>GSMSSASTFGQNAWLVDEMFQQFQKDPKSVDKEWRELFEAQGGPNTTPATTEAQPSAPKESAKPAPKAAPAAKAAPRVETKPADKTAPKAKESSVPQQPKLPEPGQTPIRGIFKSIAKNMDISLEIPTATSVRDMPARLMFENRAMVNDQLKRTRGGKISFTHIIGYAMVKAVMAHPDMNNSYDVIDGKPTLIVPEHINLGLAIDLPQKDGSRALVVAAIKETEKMNFSEFLAAYEDIVARSRKGKLTMDDYQGVTVSLTNPGGIGTRHSVPRLTKGQGTIIGVGSMDYPAEFQGASEDRLAELGVGKLVTITSTYDHRVIQGAVSGEFLRTMSRLLTDDSFWDEIFDAMNVPYTPMRWAQDVPNTGVDKNTRVMQLIEAYRSRGHLIADTNPLSWVQPGMPVPDHRDLDIETHNLTIWDLDRTFNVGGFGGKETMTLREVLSRLRAAYTLKVGSEYTHILDRDERTWLQDRLEAGMPKPTQAEQKYILQKLNAAEAFENFLQTKYVGQKRFSLEGAEALIPLMDSAIDTAAGQGLDEVVIGMPHRGRLNVLFNIVGKPLASIFNEFEGQMEQGQIGGSGDVKYHLGSEGQHLQMFGDGEIKVSLTANPSHLEAVNPVMEGIVRAKQDYLDKGVDGKTVVPLLLHGDAAFAGLGIVPETINLAKLRGYDVGGTIHIVVNNQIGFTTTPDSSRSMHYATDYAKAFGCPVFHVNGDDPEAVVWVGQLATEYRRRFGKDVFIDLVCYRLRGHNEADDPSMTQPKMYELITGRETVRAQYTEDLLGRGDLSNEDAEAVVRDFHDQMESVFNEVKEGGKKQAEAQTGITGSQKLPHGLETNISREELLELGQAFANTPEGFNYHPRVAPVAKKRVSSVTEGGIDWAWGELLAFGSLANSGRLVRLAGEDSRRGTFTQRHAVAIDPATAEEFNPLHELAQSKGNNGKFLVYNSALTEYAGMGFEYGYSVGNEDSIVAWEAQFGDFANGAQTIIDEYVSSGEAKWGQTSKLILLLPHGYEGQGPDHSSARIERFLQLCAEGSMTVAQPSTPANHFHLLRRHALSDLKRPLVIFTPKSMLRNKAAASAPEDFTEVTKFQSVINDPNVADAAKVKKVMLVSGKLYYELAKRKEKDGRDDIAIVRIEMLHPIPFNRISEALAGYPNAEEVLFVQDEPANQGPWPFYQEHLPELIPNMPKMRRVSRRAQSSTATGVAKVHQLEEKQLIDEAFEA[6x]

Contrary to most organisms in which three enzymes compose the 2-oxoglutarate dehydrogenase complex (ODH), actinobacteria rely on a two-in-one protein (OdhA) in which both the oxidative decarboxylation and succinyl transferase steps are carried out by the same polypeptide. Here we describe high-resolution cryo-EM and crystallographic snapshots of representative enzymes from Mycobacterium smegmatis and Corynebacterium glutamicum, showing that OdhA is an 800-kDa homohexamer that assembles into a three-blade propeller shape. The obligate trimeric and dimeric states of the acyltransferase and dehydrogenase domains, respectively, are critical for maintaining the overall assembly, where both domains interact via subtle readjustments of their interfaces. Schematic illustration of the reaction steps involved in the oxidative decarboxylation of 2-oxoglutarate with generation of succinyl-CoA and NADH/H+ (ODH reaction), with emphasis on the catalytic steps catalyzed by OdhA. These include the ThDP-dependent decarboxylation of the 2-oxoglutarate substrate followed the reductive acylation of the lipoyl group provided by E2p (both catalyzed by the OdhA E1o domain), and the transfer of the succinyl moiety to the CoASH acceptor (catalyzed by the OdhA E2o domain).

The same grid preparation strategy was then applied to other full-length OdhA samples, i.e. enzyme without added ligands, or preincubated with either CoASH or succinyl-CoA, leading to maps at comparable resolutions of 2.1-2.2 Å. In all cases, the maps, which showed well-defined density for most side chains, allowed to trace the OdhA polypeptide chain unambiguously starting from residue Pro102, corresponding to the N-terminal boundary of the E2o domain, with excellent stereochemical parameters. In contrast, the full N-terminal OdhA segment, corresponding to the first hundred residues that include a predicted helical hairpin analogous to the one observed in the crystal structure of MsKGD, could not be traced due to the lack of supporting density, confirming its high mobility in solution. The E1o active site at the dimer interface showed a clear density for ThDP-Mg2+ in all cases. In contrast to the crystallographic structure of OdhAΔ97 which fits the resting state, all our models refined on single particle EM maps adopt an activated conformational state of the E1o domain, even in the absence of added ligands. The state is indeed revealed by the shifts in the loops 566-579 as well as 809-836, that could be traced in the EM structures but were mostly unstructured in the OdhAΔ97 crystal structure (Fig. 3d/e). The presence of a bound acetyl-CoA activator, most likely acquired following heterologous overexpression of the enzyme in E. coli, may therefore explain the observed OdhA activated conformation through a mechanism that involves the stabilization of the loop 809-836 in its extended form, promoting, in turn, the activated conformation.> MFFSQVLRSSARAAPIKRYTGGRIGESWVITEGRRLIPEIFQWSAVLSVCLGWPGAVYF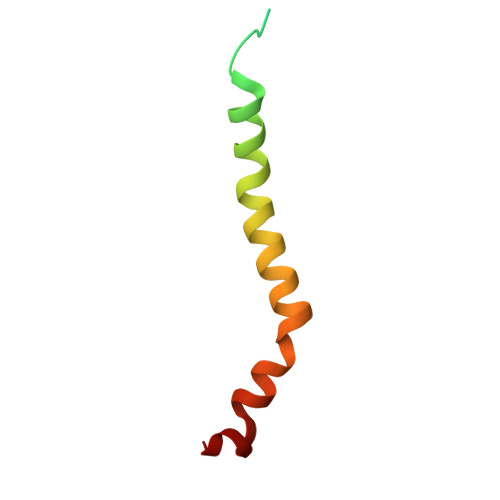FSKARKA> ATVATVNGKSISDTEVSEFFAPMLRGQDFKTLPDNQKKALIQQYIMQDLILQDAKKQNLEKDPLYTKELDRAKDAILVNVYQEKILNTIKIDAAKVKAFYDQNKDKYVKPARVQAKHILVATEKEAKDIINELKGLKGKELDAKFSELAKEKSIDPGSKNQGGELGWFDQSTMVKPFTDAAFALKNGTITTTPVKTNFGYHVILKENSQAKG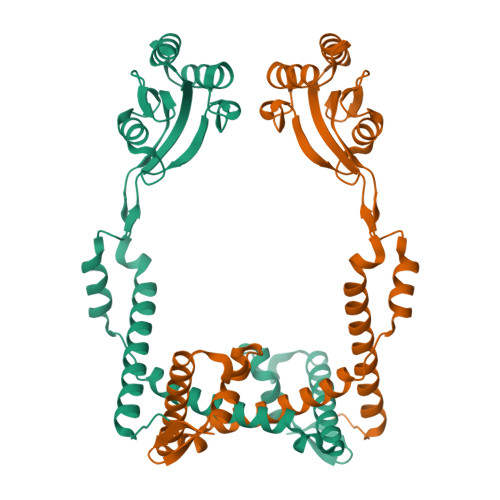QIKFDEVKQGIENGLKFEEFKKVINQKGQDLLNSAKVEYK(2R,5R)-hexane-2,5-diol | 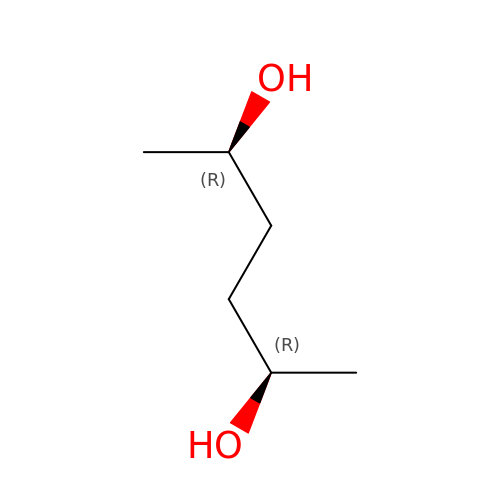C6 H14 O2 | OHMBHFSEKCCCBW-PHDIDXHHSA-N>MTIGIDKISFFVPPYYIDMTALAEARNVDPGKFHIGIGQDQMAVNPISQDIVTFAANAAEAILTKEDKEAIDMVIVGTESSIDESKAAAVVLHRLMGIQPFARSFEIKEGCYGATAGLQLAKNHVALHPDKKVLVVAADIAKYGLNSGGEPTQGAGAVAMLVASEPRILALKEDNVMLTQDIYDFWRPTGHPYPMVDGPLSNETYIQSFAQVWDEHKKRTGLDFADYDALAFHIPYTKMGKKALLAKISDQTEAEQERILARYEESIIYSRRVGN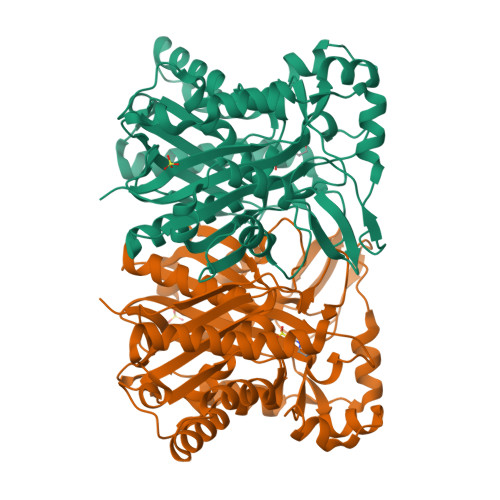LYTGSLYLGLISLLENATTLTAGNQIGLFSYGSGAVAEFFTGELVAGYQNHLQKETHLALLDNRTELSIAEYEAMFAETLDTDIDQTLEDELKYSISAINNTVRSYRN[2x]> MDFTTLQNDFTNDYQKALIANNEFLEAKKYYNGNQLPQDVLNIILERGQTPIIENMFKVIVNKILGYKIESISEIRLSPKQEEDRALSDLLNSLLQVFIQQENYDKSMIERDKNLLIGGLGVIQLWVSQDKDKNVEIEIKAIKPESFVIDYFSTDKNALDARRFHKMLEVSEQEALLLFGDSVIVNYSNVNHERIASVIESWYKEYNEETQSYEWNRYLWNRNTGIYKSEKKPFKNGACPFIVSKLYTDELNNYYGLFRDIKPMQDFINYAENRMGNMMGSFKAMFEEDAVVDVAEFVETMSLDNAIAKVRPNALKDHKIQFMNNQADLSALSQKAEQKRQLLRLLAGLNDESLGMAVNRQSGVAIAQRKESGLMGLQTFLKATDDMDRLIFRLAVSFICEYFTKEQVFKIVDKKLGDRYFKINSNDDNKIRPLKFDLILKSQLKTESRDEKWYNWNELLKILAPIRPDLVPSLVPLMLNDMDSPITNDVLEAIQNANALQQQNAEANAPYNQQIQALQIQKLQAEIMELQAKAHKYAEQGALSQTTNESEKINQAVAITE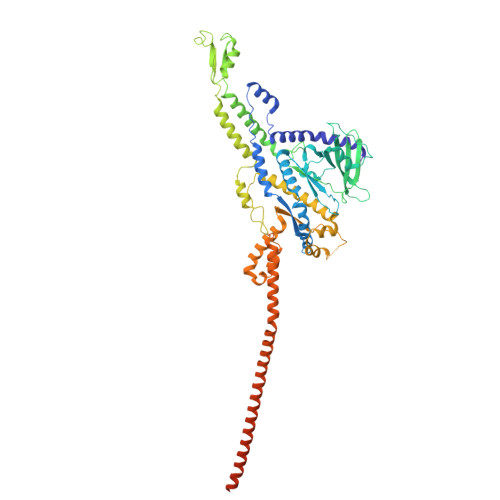MQQQNANNANNEESNNKPKKKLKTSDKTTWRKYPSAQNLDY>MRDHRKIGKQLDLYHMQEEAPGMVFWHNDGWTIFRELEVFVRSKLKEYQYQEVKGPFMMDRVLWEKTGHWDNYKDAMFTTSSENREYCIKPMNCPGHVQIFNQGLKSYRDLPLRMAEFGSCHRNEPSGSLHGLMRVRGFTQDDAHIFCTEEQIRDEVNGCIRLVYDMYSTFGFEKIVVKLSTRPEKRIGSDEMWDRAEADLAVALEENNIPFEYQLGEGAFYGPKIEFTLYDCLDRAWQCGTVQLDFSLPSRLSASYVGEDNERKVPVMIHRAILGSMERFIGILTEEFAGFFPTWLAPVQVVIMNITDSQSEYVNELTQKLSNAGIRVKADLRNEKIGFKIREHTLRRVPYMLVCGDKEVESGKVAVRTRRGKDLGSMDVNEVIEKLQQEIRSRSLKQLEEL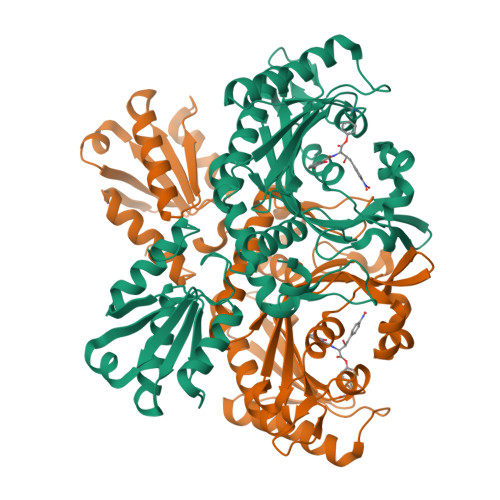EHHHHHH[2x]(5aR,9aR)-2-chloro-11-(4-beta-D-glucopyranuronosylpiperazin-1-yl)-5a,6,9,9a-tetrahydrodibenzo[b,f][1,4]oxazepine 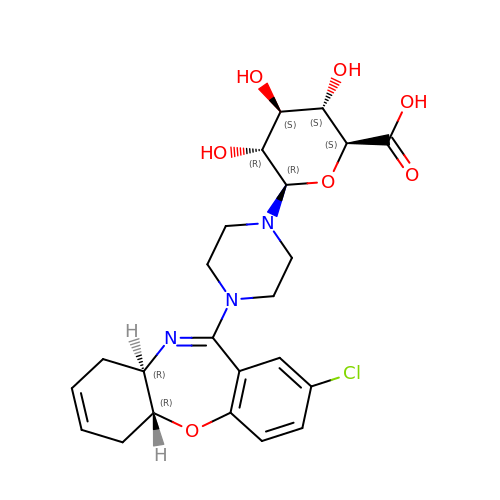| C23 H28 Cl N3 O7 | OXNRDDVCZKYHOL-IBISMJPWSA-N>[6x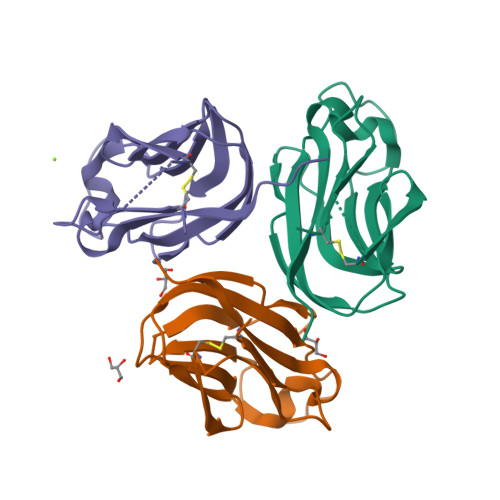]MAKDPCVAKFGPSPSEWQMASSESSCLNKMSDWKLRILQNGLYAIYGRVTPNPTYKGFAPFEVQLCKNKDAIQTLTDSSKIQNLGNIYEFNAGDTIELRFNSDDQVLKTNTYFGIILLANPQFGS N-{5-[(6,7-dimethoxyquinolin-4-yl)oxy]pyridin-2-yl}-1-methyl-3-oxo-2-phenyl-5-(pyridin-4-yl)-2,3-dihydro-1H-pyrazole-4-carboxamide 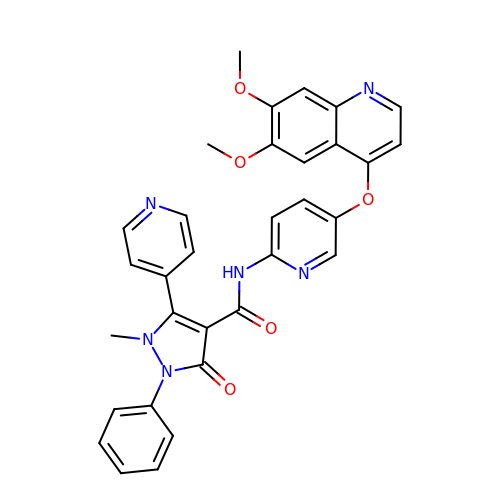| C32 H26 N6 O5 | JZUVVTPSJAHDMJ-UHFFFAOYSA-N> YDPDQYSIEADKKFKYSVKLSDYPTLQDAASAAVDGLLIDRDYNFYGGETVDFGGKVLTIECKAKFIGDGNLIFTKLGKGSRIAGVFMESTTTPWVIKPWTDDNQWLTDAAAVVATLKQSKTDGYQPTVSDYVKFPGIETLLPPNAKGQNITSTLEIRECIGVEVHRASGLMAGFLFRGCHFCKMVDANNPSGGKDGIITFENLSGDWGKGNYVIGGRTSYGSVSSAQFLRNNGGFERDGGVIGFTSYRAGESGVKTWQGTVGSTTSRNYNLQFRDSVVIYPVWDGFDLGADTDMNPELDRPGDYPITQYPLH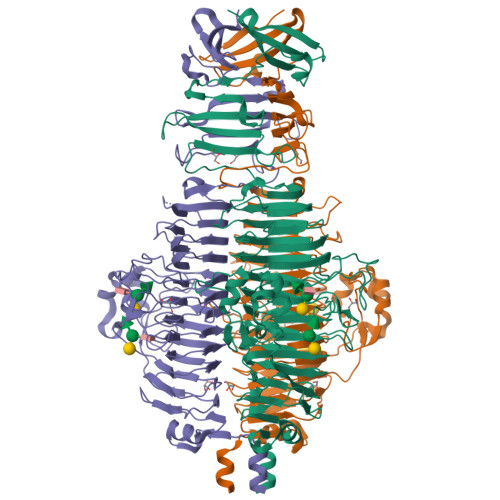QLPLNHLIDNLLVRGALGVGFGMDGKGMYVSNITVEDCAGSGAYLLTHESVFTNIAIIDTNTKDFQANQIYISGACRVNGLRLIGIRSTDGQSLTIDAPNSTVSGITGMVDPSRINVANLAEEGLGNIRANSFGYDSAAIKLRIHKLSKTLDSGALYSHINGGAGSGSAYTQLTAISGSTPDAVSLKVNHKDCRGAEIPFVPDIASDDFIKDSSCFLPYWENNSTSLKALVKKPNGELVRLTLATL> MRNEMHLQFSARSENESFARVTVAAFVAQLDPTMDELTEIKTVVSEAVTNAIIHGYNNDPNGIVSISVIIEDGVVHLTVRDEG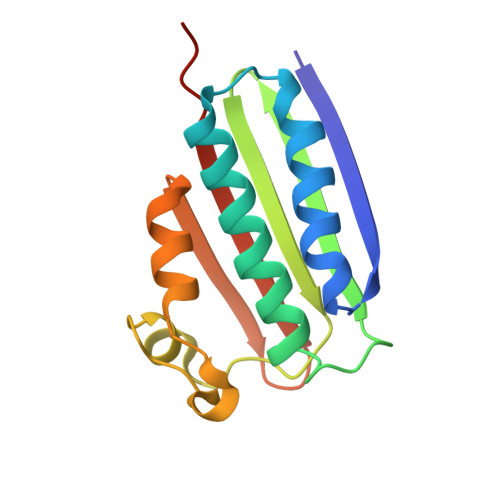VGIPDIEEARQPLFTTKPELERSGMGFTIMENFMDEVIVESEVNKGTTVYLKKHIVKSKALSN> 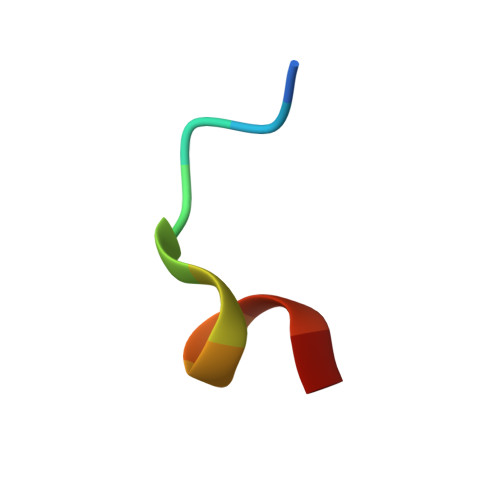ECEETEVDQHV>MDSTKEKCDSYKDDLLLRMGLNDNKAGMEGLDKEKINKIIMEATKGSRFYGNELKKEKQVNQRIENMMQQKAQITSQQLRKAQLQVDRFAMELEQSRNLSNTIVHIDMDAFYAAVEMRDNPELKDKPIAVGSMSMLSTSNYHARRFGVRAAMPGFIAKRLCPQLIIVPPNFDKYRAVSKEVKEILADYDPNFMAMSLDEAYLNITKHLEERQNWPEDKRRYFIKMGSSVENDNPGKEVNKLSEHERSISPLLFEESPSDVQPPGDPFQVNFEEQNNPQILQNSVVFGTSAQEVVKEIRFRIEQKTTLTASAGIAPNTMLAKVCSDKNKP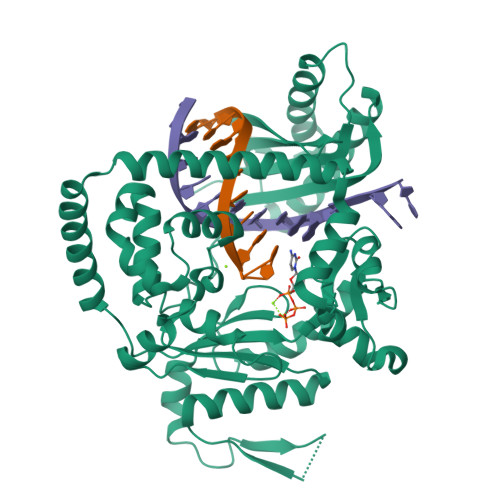NGQYQILPNRQAVMDFIKDLPIRKVSGIGKVTEKMLKALGIITCTELYQQRALLSLLFSETSWHYFLHISLGLGSTHLTRDGERKSMSVERTFSEINKAEEQYSLCQELCSELAQDLQKERLKGRTVTIKLKNVNFEVKTRASTVSSVVSTAEEIFAIAKELLKTEIDADFPHPLRLRLMGVRISSFPNEEDRKHQQ[2x]>[6x]MNKLVGLLVSSLFLASILIGIAPAITTTALTPPVSAGGIQAYLLTGSGAPASGLVLFVVNVSNIQVSSSNVTNVISTVVSNIQINAKTENAQTGATTGSVTVRFPTSGYNAYYDSVDKVVFVVVSFLYPYTTTSVNIPLSYLSKYLPGLLTAQPYDETGAQVTSVSSTPFGSLIDTSTGQQILGTNPVLTSYNSYTTQANTNMQEGVVSGTLTSFTLGGQSFSGSTVPVILYAPFIFSNSPYQAGLYNPMQVNGNLGSLSSEAYYHPVIWGRALINTTLIDTYASGSVPFTFQLNYSVPGPLTINMAQLAWIASINNLPTSFTYLSYKFSNGYESFLGIISNSTQLTAGALTINPSGNFTINGKKFYVYLLVVGSTNSTTPVEYVTKLVVEYPSSTNFLPQGVTVTTSSNKYTLPVYEIGGPAGTTITLTGNWYSTPYTVQITVGSTPTLTNYVSQILLKAVAYEGINVSTTQSPYYSTAILSTPPSEISITGSSTITAQGKLTATSASATVNLLTNATLTYENIPLTQYSFNGIIVTPGYAAINGTTAMAYVIGALYNKTSDYVLSFAGSQEPMQVMNNNLTEVTTLAPFGLTLLAPSVPATETGTSPLQLEFFTVPSTSYIALVDFGLWGNLTSVTVSAYDTVNNKLSVNLGYFYGIVIPPSISTAPYNYQNFICPNNYVTVTIYDPDAVLDPYPSGSFTTSSLPLKYGNMNITGAVIFPGSSVYNPSGVFGYSNFNKGAAVTTFTYTAQSGPFSPVALTGNTNYLSQYADNNPTDNYYFIQTVNGMPVLMGGLSIVASPVSASLPSSTSSPGFMYLLPSAAQVPSPLPGMATPNYNLNIYITYKIDGATVGNNMINGLYVASQNTLIYVVPNGSFVGSNIKLTYTTTDYAVLHYFYSTGQYKVFKTVSVPNVTANLYFPSSTTPLYQLSVPLYLSEPYYGSPLPTYIGLGTNGTSLWNSPNYVLFGVSAVQQYLGFIKSISVTLSNGTTVVIPLTTSNMQTLFPQLVGQELQACNGTFQFGISITGLEKLLNLNVQQLNNSILSVTYHDYVTGETLTATTKLVALSTLSLVAKGAGVVEFLLTAYPYTGNITFAPPWFIAENVVKQPFMTYSDLQFAKTNPSAILSLSTVNITVVGLGGKASVYYNSTSGQTVITNIYGQTVATLSGNVLPTLTELAAGNGTFTGSLQFTIVPNNTVVQIPSSLTKTSFAVYTNGSLAIVLNGKAYSLGPAGLFLLPFVTYTGSAIGANATAIITVSDGVGTSTTQVPITAENFTPIRLAPFQVPAQVPLPNAPKLKYEYNGSIVITPQQQVLKIYVTSILPYPQEFQIQAFVYEASQFNVHTGSPTAAPVYFSYSAVRAYPALGIGTSVPNLLVYVQLQGISNLPAGKYVIVLSAVPFAGGPVLSEYPAQLIFTNVTLTQ

Surface layers (S-layers) are resilient two-dimensional protein lattices that encapsulate many bacteria and most archaea. In archaea, S-layers usually form the only structural component of the cell wall and thus act as the final frontier between the cell and its environment. Sulfolobus acidocaldarius is a hyperthermophilic and acidophilic Crenarchaeon and thrives in acidic thermal soils and hot springs worldwide. The Sulfolobales S-layer lattice stands out from others because it is a two-component lattice, consisting of the S-layer-forming SlaA and the membrane anchor SlaB.

To address this knowledge gap, we performed cryoET and subtomogram averaging (STA) on S. acidocaldarius exosomes with improved imaging conditions and processing techniques. Exosomes are naturally secreted S-layer-encapsulated vesicles, with a diameter of about 90–230 nm. To analyse the in situ structure of the S-layer, we performed STA using Warp, Relion 3.1, and M and obtained a cryoEM map at 11.2 Å resolution (Figure 4—figure supplements 1 and 2). We fitted our structure of SlaA into the S-layer map, which provided an atomic model of the assembled lattice. SlaA assembles into a sheet with a thickness of 95 Å. The long axes of the SlaA subunits are inclined by an angle of about ~28° with respect to the curved S-layer surface. As a result of this inclination, effectively two zones in the SlaA assembly can be distinguished: an outer zone consisting of D1, D2, D3, and D4, and an inner zone formed by D5 and D6. Six SlaA monomers assemble around a hexagonal pore of 48 Å in diameter (glycans not included). The D1 domains of these six monomers project into and define the shape of the hexagonal pore, together with the domains D3 and D4. The D3 domain of each monomer overlaps with the D4 domain of the following monomer along the hexagonal ring in a clockwise fashion. The triangular pores that surround the hexagonal pores have a diameter of ~85 Å and are defined by the D2, D4, D5, and D6 domains of three SlaA molecules.>[2x]MAKKTSSKGKLPPGPSPLPVLGNLLQMDRKGLLRSFLRLREKYGDVFTVYLGSRPVVVLCGTDAIREALVDQAEAFSGRGKIAVVDPIFQGYGVIFANGERWR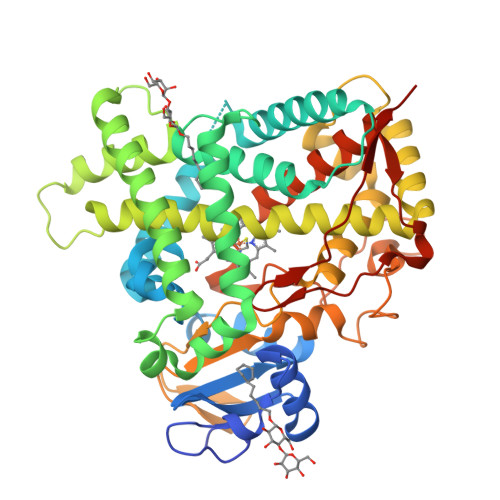ALRRFSLATMRDFGMGKRSVEERIQEEARCLVEELRKSKGALLDNTLLFHSITSNIICSIVFGKRFDYKDPVFLRLLDLWFQSFSLISSFSSQVFELFSGFLKYFPGTHRQIYRNLQEINTFIGQSVEKHRATLDPSNPRDFIDVYLLRMEKDKSDPSSEFHHQNLILTVLSLFFAGTETTSTTLRYGFLLMLKYPHVTERVQKEIEQVIGSHRPPALDDRAKMPYTDAVIHEIQRLGDLIPFGVPHTVTKDTQFRGYVIPKNTEVFPVLSSALHDPRYFETPNTFNPGHFLDANGALKRNEGFMPFSLGKRICLGEGIARTELFLFFTTILQNFSIASPVPPEDIDLTPRESGVGNVPPSYQIRFLARHHHHHH>MKYDTSELCDIYQEDVNVVEPLFSNFGGRASFGGQIITVKCFEDNGLLYDLLEQNGRGRVLVVDGGGSVRRALVDAELARLAVQNEWEGLVIYGAVRQVDDLEELDIGIQAMAAIPVGAAGEGIGESDVRVNFGGVTFFSGDHLYADNTGIILSEDPLDIE[3x];> RKKIHQWYYRADDLEHKTALLVHLLKQPEATRSIVFVRKRERVHELANWLREAGINNCYLEGEMVQGKRNEAIKRLTEGRVNVLVATDVAARGIDIPDVSHVFNFDMPRSGDTYLHRIGRTARAGRKGTAISLVEAHDHLLLGKVGRYIEEPIKARVIDELRPKTRAPSE

As an inhibitor of RNase E, RraA has widespread effects on transcript levels in E. coli, although its physiological role in ribonuclease regulation is debated. Surprisingly, in vitro RraA does not inhibit the catalytic activity of RNase E directly, but appears to act indirectly by occluding RNA binding regions in the C-terminal domain of the ribonuclease. We have previously shown that RraA can directly interact with RhlB, and it is possible that RraA plays two distinct roles in modulating the degradosome, by inhibiting both its ribonuclease and helicase activities. We present biochemical and structural data to characterize the interaction between RraA and SrmB, and provide structural data on the interaction of RhlB with RraA and compare the two complexes.

The crystallographic asymmetric unit contains a single torus-shaped trimer of RraA bound to one SrmB RecA-like α/β sandwich domain. Following close inspection of the electron density maps it was clear that the RecA-like domain resolved in the crystal structure corresponds to the CTD of SrmB (residues 219–388). The CTD has a typical DEAD-box protein-fold and engages the outside rim of the RraA trimer, such that only one RraA protomer is engaged with the SrmB CTD. There are no significant structural changes in the RraA protomer that contacts the SrmB CTD compared with the two protomers not bound to SrmB. The last 56 residues of SrmB corresponding to the CTE, which are predicted to be natively unstructured, were also not resolved in the final model, and this may indicate that this region is indeed disordered. Inspection of the interface between SrmB and RraA reveals electrostatic complementarity formed by a positively charged patch on SrmB and a negatively charged cluster on RraA. The interface involves mainly salt bridging interactions of side chains and hydrogen bonds between main chain atoms. Most of the RraA residues involved in the interaction with SrmB are conserved and two of these residues (Asp-50 and Glu-53) were predicted earlier to be involved in RraA interactions with other proteins. Closer inspection of the superimposed helicase structures reveals that bound RraA partially occludes the RNA binding surface of SrmB. Based on these structural overlays, we propose that RraA can influence SrmB activity by sterically inhibiting substrate binding and preventing the enzyme from adopting the closed conformation required for ATP hydrolysis.>ATTYIFGKGGALITYTWPPNDRPSTRMDRLAVGFSTHQRSAVLVRVDSASGLGDYLQLHIDQGTVGVIFNVGTDDITIDEPNAIVSDGKYHVVRFTRSGGNATLQVDSWPVNERYPAGRQLTIFNSQAAIKIGGRDQGRPFQGQVSGLYYN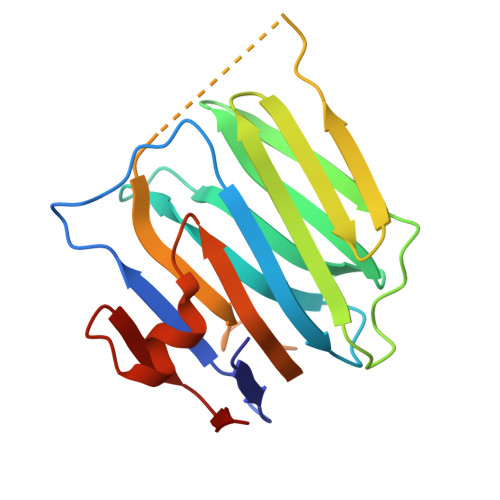GLKVLALAAESDPNVRTEGHLRLV[3x]> MACLSPSQLQKFQQDGFLVLEGFLSAEECVAMQQRIGEIVAEMDVPLHCRTEFSTQEEEQLRAQGSTDYFL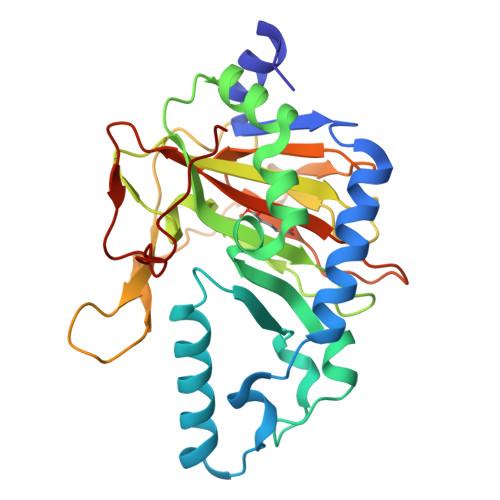SSGDKIRFFFEKGVFDEKGNFLVPPEKSINKIGHALHAHDPVFKSITHSFKVQTLARSLGLQMPVVVQSMYIFKQPHFGGEVSPHQDASFLYTEPLGRVLGVWIAVEDATLENGCLWFIPGSHTSGVSRRMVRAPVGSAPGTSFLGSEPARDNSLFVPTPVQRGALVLIHGEVVHKSKQNLSDRSRQAYTFHLMEASGTTWSPENWLQPTAELPFPQLYT>[2x]MSTSSSSQSLKIGIVGFGNFGQFLAKTMIKQGHTLTATSRSDYSELCLQMGIHFFRDVSAFLTADIDVIVLCTSILSLSEVVGSMPLTSLKRPTLFVDVLSVKEHPRELLLRELPEDSDILCTHPMFGPQTAKNGWTDHTFMYDKVRIRDEVICSNFIQIFATEGCKMVQMSCEEHDRAAAKSQFITHTIGRTLGEMDIQSTPIDTKGFETLVKLKETTMRDSFDLYSGLFVYNRFARQELENLEH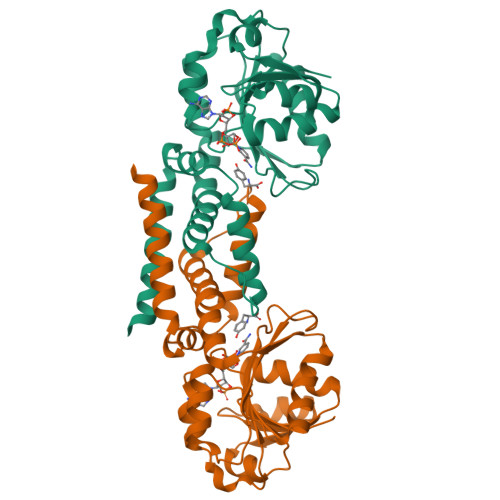ALHKVKETLMIQRTNGEQGHKRTES>GQDMVSPPPPIADEPLTVNTGIYLIESYSLDDKAETFKVNAFLSLSWKDRRLAFDPVRSGVRVKTYEPEAIWIPEIRFVNVENARDADVVDISVSPDGTVQYLERFSARVLSPLDFRRYPFDSQTLHIYLIVRSCDTRNIVLAVDLEKVGKNDDVFLTGWDIESFTAVVKPANFALEDRLESKLDYQLRISRQYFSYIPNIILPMLFILFISWTAFWSTSYEANVTLVVSTLIAHIAFNILVETNLPKTPYMTYTGAIIFMIYLFYFVAVIEVTV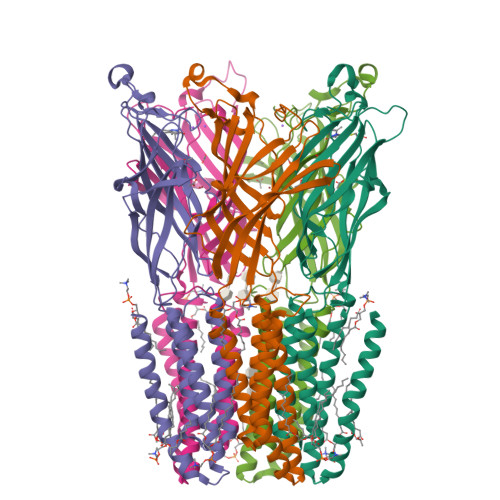QHYLKVESQPARAASITRASRIAFPVVFLLANIILAFLFFGF[5x]> GHMDLIRSADIQMRELSRL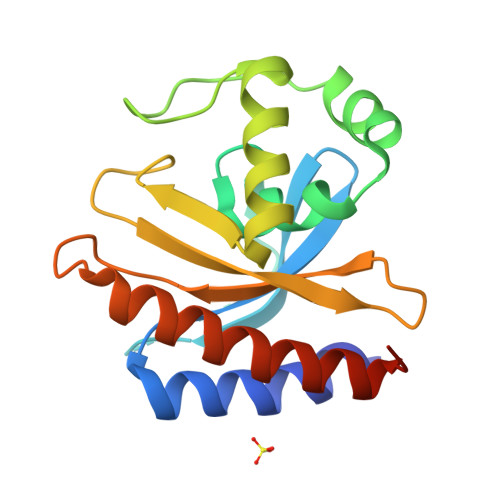TKETIHLGALDEDSIVYIHKIDSMYNLRMYSRIGRRNPLYSTAIGKVLLAWRDRDEVKQILEGVEYKRSTERTITSTEALLPVLDQVREQGYGEDNEEQEEGLRCIAVPVFDRFGVVIAGLSISFPTLRFSEERLQEYVAMLHTAARKISAQMGYHDYPFGS> KQKPRYEIRWRVIESISPDGHEYIYVDPMQLPYDSRWEFPR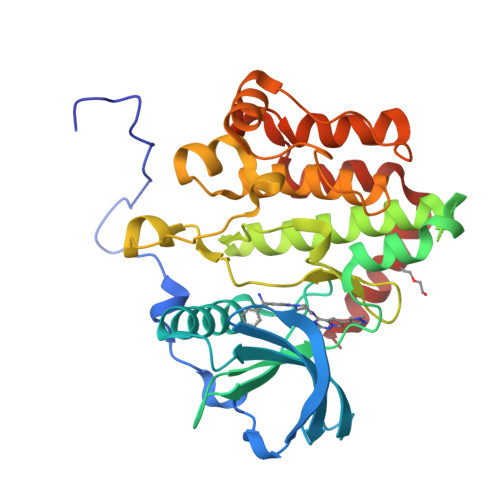DGLVLGRVLGSGAFGKVVEGTAYGLSRSQPVMKVAVKMLKPTARSSEKQALMSELKIMTHLGPHLNIVNLLGACTKSGPIYIIIEYCFYGDLVNYLHKNRDSFLSHKKKSMLDSEVKNLLSDDNSEGLTLLDLLSFTYQVARGMEFLASKNCVHRDLAARNVLLAQGKIVKICDFGLARDIMHDSNYVSKGSTFLPVKWMAPESIFDNLYTTLSDVWSYGILLWEIFSLGGTPYPGMMVDSTFYNKIKSGYRMAKPDHATSEVYEIMVKCWNSEPEKRPSFYHLSEIVENLLPGQYKKSYEKIHLDFLKSD>[4x]MTSPSSPPAFRLETSDGGQDGAEVDKAQLGYGAGPPPMESRFQDEDRNFPPQIKVNLNYRKGAGASQPDLNRFDRDRLFNVVARGNPEDLAGLLEYLRRTSKYLTDSEYTEGSTGKTCLMKAVLNLQDGVNACIQPLLEIDRDSGNPQPLVNAQCTDEYYRGHSALHIAIEKRSLQCVKLLVENGANVHAKACGHFFQKNQDTCFYFGELPLSLAACTKQWDVVNYLLENPHQPASLQAQDSLGNTVLHALVMIADDSAENSALVVRMYDGLLQAGARLCPNVQLEGIPNLEGLTPLKLAAKEGKIEIFKHILQREFSAPCQSLSRKFTEWCYGPVRVSLYDLASVDSWEENSVLEIIAFHSRSPHRHRM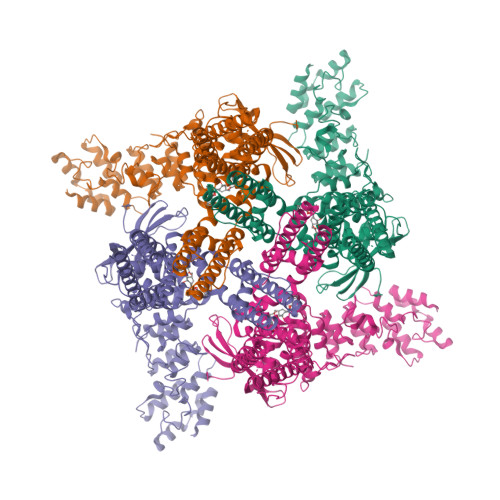VVLEPLNKLLQAKWDRLIPRFCFNFLCYLVYMLIFTAVAYHQPALEKQGFPPLKATAGNSMLLLGHILILLGGVYLLLGQLWYFWRRRLFIWISFMDSYSEILFLLQALLTVLSQVLCFLAIEWYLPLLVSSLAMGWTNLLYYTRGFQHTGIYSVMIEKVILRDLLRFLLVYLVFLFGFAVALVSLSREAQNSRTPAGPNATEVGQPGAGQEDEAPPYRSILDASLELFKFTIGMGELAFQEQLRFRGVVLLLLLAYVLLTYVLLLNMLIALMSETVNSVATDSWSIWKLQKAISVLEMENGYWWCRRKKQRAGVMLTVGTRPDGSPDERWCFRVGEMNWATWEQTLPRTLCEEPSGAAAPGVMKNPTPASQRGEDSASEEDHLPLQLLQSRSNLEVLFQGPHHHHHHDYKDDDDK>[2x]DAAQPARRANGSEWSYTNILTGPETWHEHYKNMCSGYYQSPIDLKTDISTLDLKLKTVIIYRNTSSTETTTIQNNGHSAEVKFPRNTWFISFDGILDYKYEIIQMHFHWGNTDDRGSEHTIDGFRFPLEGHIVSFRRQMYSSPSEAIGRPGGLAVLGIMHQIVESIKYEQTAFKAYNNFSGVLNS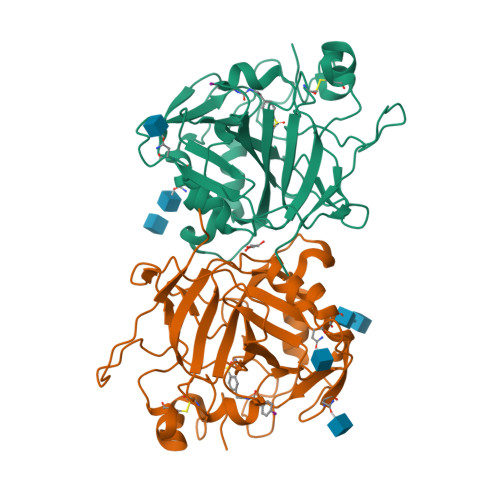QFVPPNNSTIDDINLALLLSLLNPSRYFRYLGSLTTPPCTENVLWTVFIDPVLITREQINLFRNLPYGSNEKQTRMGDNFRPIQLLNPIDTLASRTLYRATARGGPEQKLISEEDLNSAVDHHHHHH GUANOSINE-5'-DIPHOSPHATE-RHAMNOSE | C16 H25 N5 O15 P2 | 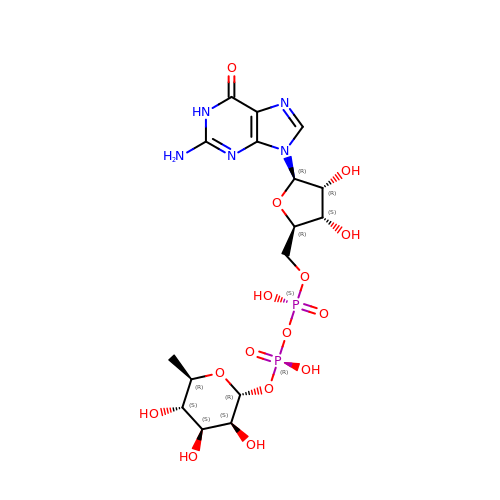LQEBEXMHBLQMDB-GDJBGNAASA-N>[2x]MPGSKPTKTEEEDDPTPYLFVSLEQKRIDQTKPYDAKKACWVPDEHEGFVQGEIRGTKGDIVSVHLPNGETKDFKKDQVGQVNPPKFEKCEDMSNLTYLNDASVLYNLKQRYYNKLIYTYSGLFCVAINPYKRFPVYTMRCAKLYRGKRRNEVPPHIFAISDGAYVNMLTNKENQSMLITGESGAGKTENTKKVIAYFATVGASTKKEEAASAASQKKGTLEDQVVQTNPVLEAFGNAKTVRNDNSSRFGKFIRIHFGPSGKLAGADIETYLLEKARVISQQSLERSYHIFYQVMSGAVPGVKELCLLSNDIYEYNYVSQGKVTIPSVDDGEEFQATDQAFDVLGFTQEEKDDIYKITASVMHMGCMKFKQRGREEQAEADGTAEGERVAKLLGLEAADLYKNLLKPRIKVGNEFVTQGRNLNQVIYSVGALSKGVFDRLFKFLVKKCNETLDTKQKRQHFIGVLDIAGFEIFDFNGFEQLCINFTNEKLQQFFNHHMFVLEQEEYTREGITWAFIDFGMDLVACIDLIEKPMGILSILEEESMFPKATDKTFEEKLMNNHLGKSPNFQKPKPPKPGCQAAHFAISHYAGVVSYNLTGWLEKNKDPLNDTVVDQFKKGSNKLLVEIFADHPGQSGAPEAGGGGKGGRGKKGGGFATVSSSYKEQLNNLMTTLKSTQPHFVRCIIPNELKQPGLIDSHLVMHQLTCNGVLEGIRICRKGFPNRMVYPDFKLRYMILAPATMAAEPDPKKAADKCLKEVGLESETYRIGHTKVFFRAGVLGQLEEMRDERLSKIIGWMQSHIRGYLARKQFKKYQDQRLSLQVVQRNLRKYMALRTWPWWKMWTKVKPLLNVANVEEEMRKLEELVATTQAALEKEEKARKEVEALNAKLIQEKTDLLRNLEGEKGSISSIQEKAAKLQAQKSDLESQLMDTQERLQQEEDN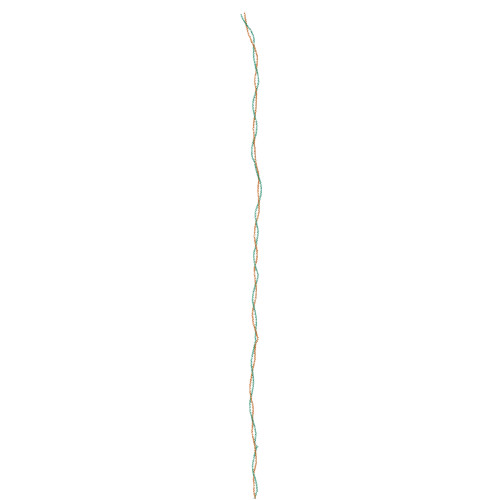RNQMFQQKKKLEQEVGGLKKDIEDLELSLQKSDQDKASKDHQIRNLNDEIAHQDELINKLNKEKKMQGEHTQKTAEELQASEDKVNHLTKVKAKLEQTLDELEDSLEREKKLRGDVEKAKRKVEGDLKLTQEAVADLERNKKELEQTIQRKDKEIASLTAKLEDEQSIVSKTQKQIKELQSRIEELEEEVEAERQARGKAEKQRADLARELEELGERLEEAGGATSAQIELNKKREAEMSKLRRDLEESNIQHESTLANLRKKHNDAVSEMGEQIDQLNKLKTKAEHDRTHVQNDLNNTRHALDQMCREKAATEKIAKQLQHQVNEIQGKLDEANRTLNDFDSAKKKLSIENSDLLRQLEEAESQVSQLSKIKVSLTTQLEDTKRLADEEARERATLLGKFRNLEHDLDNIREQLEEEAEGKADIQRQLSKANAEAQLWRTKYESEGVARAEELEEAKRKLQARLAEAEETIESLNQKVIALEKTKQRLATEVEDLQLEVDRATAIANAAEKKAKAIDKIIGEWKLKVDDLAAELDASQKECRNYSTELFRLKGAYEEAQEQLEAVRRENKNLADEVKDLLDQIGEGGRNIHEIEKQKKRLEVEKDELQAALEEAEAALEQEENKVLRSQLELSQVRQEIDRRIQEKEEEFENTRKNHQRALDSMQASLEAEAKGKAEALRMKKKLEADINELEIALDHANKANSEAQKTIKKYQQQLKDVQTALEEEQRARDDAREQLGISERRANALQNELEESRTLLEQADRGRRQAEQELGDAHEQINELAAQATSASAAKRKLEGELQTLHADLDELLNEAKNSEEKAKKAMVDAARLADELRAEQDHAQTQEKLRKALETQIKELQIRLDEAETNALKGGKKAIAKLEQRVRELENELDGEQRRHADAQKNLRKSERRIKELSFQADEDRKNHERMQDLVDKLQQKIKTYKRQIEEAEEIAALNLAKFRKAQQELEEAEERADLAEQAIAKFRTKGGRAGSAARAMSPVAHRPPVKHPLDGSTFPPRFDLHEDMM>[2x]MDNPPTFSKPAYFVSVLENIMAGATVLFLNATDLDRSREYGQESIIYSLEGSSQFRINARSGEITTTSLLDRETKSEYILIVR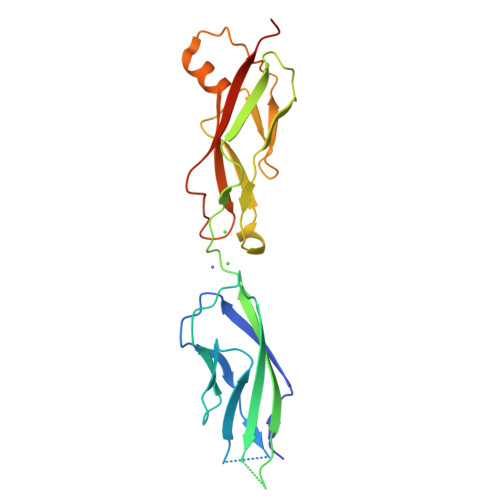AVDGGVGHNQKTGIATVNVTLLDINDNHPTWKDAPYYINLVEMTPPDSDVTTVVAVDPDLGENGTLVYSIHPPNKFYSLNSTTGKIRTTHVMLDRENPDPVEAELMRKIIVSVTDCGRPPLKATSSATVFVNLLDLNDNLEHHHHHH> APGSVVELLGKSYPQDDHSNLTRKVLTRVGRNLHNQQHHPLWLIKERVKEHFYKQYVGRFGTPLFSVYDNLSPVVTTWQNFDSLLIPADHPSRKKGDNYYLNRTHMLRAHTSAHQWDLLHAGLDAFLVVGDVYRRDQIDSQHYPIFHQLEAVRLFSKHELFAGIKDGESLQLFEQSSRSAHKQETHTMEAVKLVEFDLKQTLTRLMAHLFGDELEIRWVDCYFPFTHPSFEMEINFHGEWLEVLGCGVMEQQLVNSAGAQDRIGWAFGLGLERLAMILYDIPDIRLFWCEDERFLKQFCVSNINQKVKFQPLSKYPAVINDISFWLPSENYAENDFYDLVRTIGGDLVEKVDLIDKFVHPKTHKTSHCYRITYCHMERTLSQREVRHIHQALQEAAVQLLGVEGRF

Mutations in the mitochondrial aminoacyl‐tRNA synthetases (mtaaRSs) can cause profound clinical presentations, and have manifested as diseases with very selective tissue specificity. Among the recently reported pathogenic variants are point mutations in FARS2 gene, encoding the human mitochondrial PheRS. Patient symptoms range from spastic paraplegia to fatal infantile Alpers encephalopathy. How clinical manifestations of these mutations relate to the changes in three‐dimensional structures and kinetic characteristics remains unclear, although impaired aminoacylation has been proposed as possible etiology of diseases.

Here, we report four crystal structures of HsmtPheRS mutants, and extensive MD simulations for wild‐type and nine mutants to reveal the structural changes on dynamic trajectories of HsmtPheRS. Using steady‐state kinetic measurements of phenylalanine activation and tRNAPhe aminoacylation, we gained insight into the structural and kinetic effects of mitochondrial disease‐related mutations in FARS2 gene.>[2x]MPKLVTWMNNQRVGELTKLANGAHTFKYAPEWLASRYARPLSLSLPLQRGNITSDAVFNFFDNLLPDSPIVRDRIVKRYHAKSRQPFDLLSEIGRDSVGAVTLIPEDETVTHPIMAWEKLTEARLEEVLTAYKADIPLGMIREENDFRISVAGAQEKTALLRIGNDWCIPKGITPTTHIIKLPIGEIRQPNATLD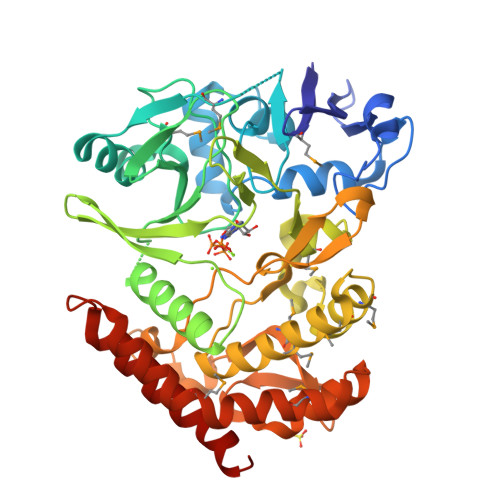LSQSVDNEYYCLLLAKELGLNVPDAEIIKAGNVRALAVERFDRRWNAERTVLLRLPQEDMCQTFGLPSSVKYESDGGPGIARIMAFLMGSSEALKDRYDFMKFQVFQWLIGATQGHAKNFSVFIQAGGSYRLTPFYDIISAFPVLGGTGIHISDLKLAMGLNASKGKKTAIDKIYPRHFLATAKVLRFPEVQMHEILSDFARMIPAALDNVKTSLPTDFPENVVTAVESNVLRLHGRLSREYGSK> MDNPNPGPDGEGEVELEKDSNVVLTTQRDPSTSIPAPVSVKWSRWTSNDVVDDYATITSRWYQIAEFVWSKDDPFDKELARL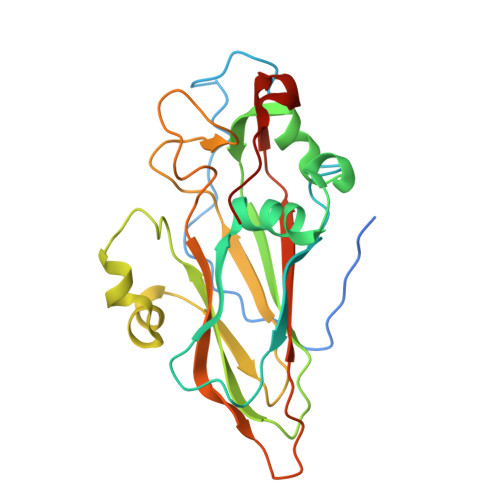ILPRALLSSIEANSDAICDVPNTIPFKVHAYWRGDMEVRVQINSNKFQVGQLQATWYYSDHENLNISSKRSVYGFSQMDHALISASASNEAKLVIPFKHVYPFLPTRIVPDWTTGILDMGALNIRVIAPLRMSATGPTTCNVVVFIKLNNSEFTGTSSGKFYASQIRAKPE> RRGLLPNHIWQGDVTHYKYKKYKYCLHVWVDTFSGAVSVSCKKKETSCETISAFLQAISLLGKPLHINTDNGPAFLSQEFQEFCTSYHIKHSTHIPYNPTSSGLVERTNGIIKNLLNKYLLDCPNLPLDNAINKALWTLNQLNVMNPSGKTRWQIHHSPPLPPIPEAST

IN first catalyses 3′-processing of the vDNA ends, exposing reactive 3′ OH nucleophile groups that it uses to attack a pair of phosphodiester bonds within target DNA (tDNA), resulting in strand transfer. In this work, we determine the three-dimensional structure of the deltaretroviral intasome and characterize its interactions with its host factor, the PP2A-B56γ subunit. The deltaretroviral IN host cofactor B56γ14, as part of the heterotrimeric protein phosphatase 2A (PP2A) holoenzyme, interacts with a number of chromatin-associated proteins and potently stimulates concerted integration activity of deltaretroviral INs14.

To aid the interpretation of the cryo-EM map, we generated a high-quality homology model of the STLV-1 IN/NTD using the SWISS-MODEL server, and determined a series of X-ray crystal structures spanning the catalytic core domain (CCD) and the C-terminal domain (CTD) of HTLV-2 and -1 IN.> QIASDVEAPPPAPAKVEKHSKKMEEGITVNKFKPKTPYVGRCLLNTKITGDDAPGETWHMVFSHEGEIPYREGQSVGVIPDGEDKNGKPHKLRLYVIASSALGDFGDAKSVSLCVKRLIYTNDAGETIKGVCSNFLCDLKPGAEVKLTGPVGKEMLMPKDPNATIIMLGTGTGIAPFRSFLWKMFFEKHDDYKFNGLAWLFL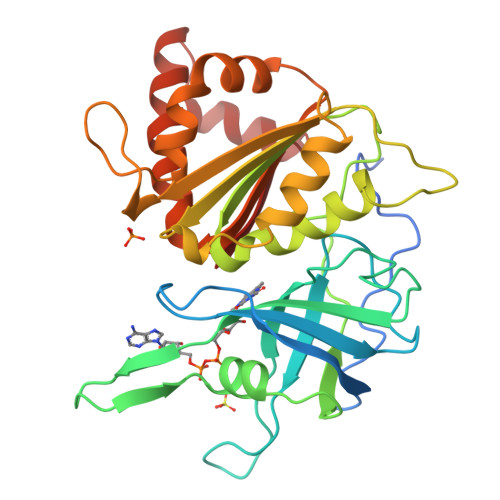GVPTSSSLLYKEEFEKMKEKAPDNFRLDFAVSREQTNEKGEKMYIQTRMAQYAVELWEMLKKDNTYFYMCGLKGMEKGIDDIMVSLAAAEGIDWIEYKRQLKKAEQWNVEVY>[2x]MRPETIPGISLNEDNSHYFYTRAGRRLSAEEVDSWVDQYAGTQVKELMLCPNCMRTSYASQVWDPIWRGYDPAGPDDQPLLASLPPEERVAARGWIHTAWQLHQDGIDIYARWIRRCRQRGISPWISMRMNDVHYVNDERCFLHSEFWRENPQLRRVPYRFAEWTDRAFDYGRAEVREHHLKLIRELAARYDFDGLELDWMRFGFHFRPGYEAEGAEILTAFTAEVRRLLDDWEKRRGHKIHLGARIPSRPATALGLGMDAVTWARRGLVDMLVITPFWASAETDMPVEIWRQLLEGTGVTLAAGLEVLLRPYPDSPLFQTNSLETVRGAAASLLDRGAQRIYLFNYMDSQTAMEDLENYPTLLREIGSLETLAGKPRRHVLTFADTWAPGEPRAIPLPATCRPGEWRAFRLHTGPKPEPGEVIAALGIEGGVAIGPETLEVRVNGELCAFLGLVDLSKPRPDFPVYGFSVPLAAMRRGYNLIEVTARQELRFGWAEFLIRPWHSHHHHHH

Here we describe the 3-D structure and catalytic center of the defining member, EnvSia156, of this sialidase family. We show, through ligand complexes with products and sialidase inhibitors, that the 3-D structure and active center are indeed an unusual arrangement, with family-conserved histidine and aspartate residues defining the catalytic mechanism that acts with inversion of anomeric configuration; facets not previously observed in the canon of literature for sialidases. The catalytic domain (residues 6–376) comprises a complete (β/α)8-barrel fold while the C-terminal domain (residues 377–502) consists of an eight-stranded β-sandwich. Here we show that GH156 sialidases define a distinct paradigm for sialidase action with His and Asp acting as Brønsted acid and base, respectively, in an inverting mechanism that is unique amongst all exo-sialidases described to date.

The best model was obtained from a crystal of EnvSia156 with bound Neu5Ac (EnvSia156Neu5Ac), at a resolution of 2.0 Å. To better define, the active center residues, 3-D structures were determined with the product Neu5Ac and with the inhibitor DANA (Ki 3 μM). The structures with Neu5Ac show the β-anomer (equating to a product complex following catalytic attack on an α-sialoside with inversion) of the ligand interacting with EnvSia156 at the predicted catalytic center based on sequence homology, through 13 hydrogen bonds (with 8 more mediated by water molecules) and several hydrophobic interactions. The –1 subsite, which accommodates the sialic acid monosaccharide, shows several differences from what is commonly observed in other sialidases. It is possible to identify the characteristic triad of residues coordinating the carboxylate group, although it consists of two arginine side-chains (Arg129 and Arg202) and one asparagine (Asn346), instead of the three arginines displayed in conventional sialidases. Invariant Asp14 lies adjacent to the (anomeric) C2 carbon and makes a hydrogen bond with the hydroxyl group. Thus, Asp14 is the most likely candidate to act as a general catalytic base residue (discussed further below). The structure of EnvSia156 with Neu5Ac shows a single discrete non-bonded contact between Gln351 and the acetamide methyl group and one water-mediated hydrogen bond between N5 and Asp14/Ser16. Asp14 is ideally placed to assume the role of general base, through its position on the “beta” face and its direct interaction with the product OH in the Neu5Ac complex. When overlaying this structure with that of EnvSia156Neu5Ac it is possible to speculate that a similar process occurs, with the carboxylate held in a pseudo-equatorial orientation by Arg129, Arg202, and Asn346, and the aglycone fitting into the pocket formed by Trp164, Phe203, Phe278, and Trp279, forcing the glycosidic bond into a pseudo-axial orientation.>[14x]GMEAYLNKIDKIEPSDQKIKEEYNKFKYDITKQAIESLRERIPKRIIFFNNLVNVNSEPGSILNVNDLDGVSYKYKINKIEENVRKKHKGNN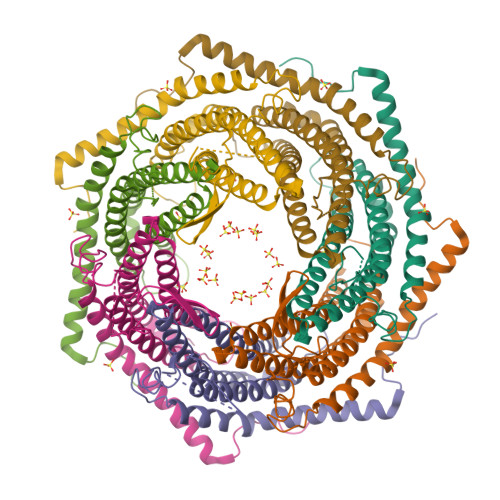SSDFDEREKKKDSLDGHVKHFSNNEDSKLIIDDKVLYTHYVPSHKQIYLELEKIKTYASELIEIIGNIKLWIQLNVPRIEDGNNFGVGIQEEAIQELARVEESAFNLYDAIVKYYMERAKISTKVLKYPNVSDYQEAVRELDEKEWIHIKITIVDMRNNYIMLYDLLYKNWEKVVKPKNEDAHHRMTF> SMADRGDSGDSDFVVVANRLPIDLERAPDGTTSWKRSPGGLVTALEPLLRRRRGAWIGWPGIPDSDEDPIVDGDLVLYPVRLSADDVAQYYEGFSNATLWPLYHDVIVKPIYNRQWWERYVEVNRRFAEATSRAAARGATVWVQDYQLQLVPKMLRELRPDLTIGFFLHIPFPPVELFMQLPWRTEITDGLLGADLVGFHLPGGAQNFLFLARRLVGANTSRASVGVRSKFGEVQIGSRTVKVGAFPISIDSADLDRQARQRSIRQRARQIRAELGNPRRILLGVDRLDYTKGIDVRLQAFAELLAEGRVNREDTVFVQLATPSRERVEAYRLLRDDIERQVGHINGEYGEVGHPVVHYLHRPVPREELIAFFVAADVMLVTPLRDGMNLVAKEYVACRSDLGGALVLSEFTGAAAELGQAYLVNPHNLDHVKDTMVAALNQTPEEGRRRMRALRRQVLAHDVDLWARSFLDALASTRTGDADAVPV

OtsA is a glycosyltransferase that uses the α anomer of G6P as acceptor and NDP-glucose as the donor to synthesize T6P. In this pathway, which is conserved and essential in mycobacteria, trehalose is synthesized in a two-step process involving OtsA and OtsB2 enzymes. MtrOtsA is composed of two Rossmann-fold domains with a deep catalytic site at their interface, in an arrangement typical of GT-B glycosyltransferases for other organisms. MtrOtsA forms a tetramer in solution, as previously observed for M. tuberculosis OtsA.

Structures with donor substrates were determined by soaking the apo form crystals with ADP-glucose and GDP-glucose. The donor substrates interact primarily with the C-terminal domain through the side chains of the highly conserved Arg286, Lys291, Asp385, and Glu393 and with the side chain of Arg365, which is conserved in all mycobacteria and closely related species but less conserved outside this group. Backbone interactions with the absolutely conserved residue Gly386, Met387, Asn388, and Leu389 amine groups are also observed. N-terminal domain interactions with the donor substrate are observed only for His168 when the active site is in an open conformation. Preference for ADP-glucose as the donor substrate in MtrOtsA is conferred by interactions with the deeply buried adenine moiety. The carbonyl groups of Leu319 and Arg361 interact with the primary amine, and the amide group of Val363 interacts with N-1 of the adenine moiety. A highly coordinated water interacts with the primary amine of the adenine moiety and the carbonyl groups of Leu359 and Arg361. The presence of the leucine in M. thermoresistibile allows the primary amine of the adenine moiety to occupy a buried position, interacting with the carbonyl group of Leu319 which no other nucleotide activated donor can occupy. The binding affinity of substrate donors could be determined only for ADP-glucose under the tested conditions with an observable Kd (dissociation constant) of 27.17 ± 2.66 μM.>MHELTIYHFMSDKLNLYSDIGNIIALRQRAKKRNIKVNVVEINETEGITFDECDIFFIGGGSDREQALATKELSKIKTPLKEAIEDGMPGLTICGGYQFLGKKYITPDGTELEGLGILDFYTESKTNRLTGDIVIESDTFGTIVGFENHGGRTYHDFGTLGHVTFGYGNN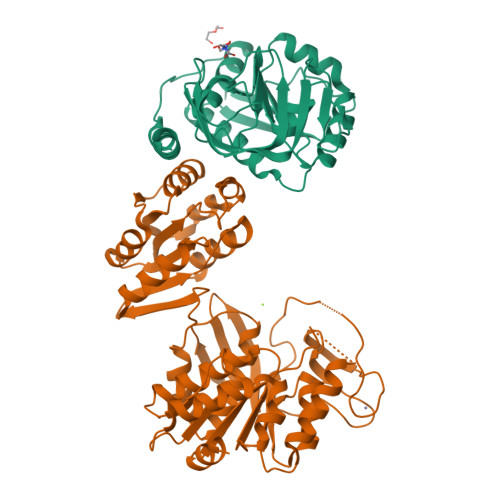DEDKKEGIHYKNLLGTYLHGPILPKNYEITDYLLEKACERKGIPFEPKEIDNEAEIQAKQVLIDRANRQKKSRLEHHHHHH[2x];>[2x]MRQWTAIHLAKLARKASRAVGKRGTDLPGQIARKVDTDVLRKLAEQVDDIVFISGTNGKTTTSNLIGHTLKANNIQIIHNNEGANMAAGITSAFIMQSTPKTKIAVIEIDEGSIPRVLKEVTPSMMVFTNFFRDQMDRFGEIDIMVNNIAETISNKGIKLLLNADDPFVSRLKIASDTIVYYGMKAHAHEFEQSTMNESRYCPNCGRLLQYDYIHYNQIGHYHCQCGFKREQAKYEISSFDVAPFLYLNINDEKYDMKIAGDFNAYNALAAYTVLRELGLNEQTIKNGFETYTSDNGRMQYFKKERKEAMINLAKNPAGMNASLSVGEQLEGEKVYVISLNDNAADGRDTSWIYDADFEKLSKQQIEAIIVTGTRAEELQLRLKLAEVEVPIIVERDIYKATAKTMDYKGFTVAIPNYTSLAPMLEQLNRSFEGGQS The Chili RNA aptamer mimics large Stokes shift fluorescent proteins and exhibits high affinity for 3,5-dimethoxy-4-hydroxybenzylidene imidazolone (DMHBI) derivatives to elicit green or red fluorescence emission. The Chili RNA folds into a single coaxial helical stack with a length of ~70 Å that contains two A-form duplexes P1 and P2 that are separated by the central fluorophore binding domain (FBD). The P1 stem transitions via a base triple into a two-tiered G-quadruplex, which constitutes the core of the FBD. The ligand is immobilized by π-stacking between an unusual G14:G31 base pair and the T2 quartet.

Likewise, the structure of Chili–DMHBI+ was solved by MR and refined at a resolution of 2.95 Å. The crystallographic asymmetric unit (ASU) of the native datasets contained four copies of RNA-ligand complexes, which were superimposable with a root mean square deviation (rmsd) of 0.3 Å. The structural features of the DMHBO+ and DMHBI+ complexes are highly similar. In contrast to Spinach, which binds the deprotonated form of DFHBI, Chili exclusively binds the phenol form of DMHBI derivatives but enhances fluorescence of the phenolate forms. The positively charged groups in DMHBI+ and DMHBO+ substantially enhanced the binding affinity and fluorescence brightness. Time-correlated single photon counting (TCSPC) on the ns timescale revealed multiexponential decays for both Chili–DMHBO+ and Chili–DMHBI+ complexes but did not resolve the kinetics of proton transfer. Fluorescence and TA measurements on Chili–DMHBI+ gave a similar picture although with transient spectra shifted to shorter wavelengths. Again, proton transfer occurred in 120 fs. Preliminary 2D NMR experiments of the Chili–DMHBI+ complex in K+/Mg2+ solution revealed an unusual signal at a proton chemical shift of 8.6 ppm and 15N chemical shift of 142 ppm. The resonance unambiguously arises from an exchangeable proton of a guanine but does not belong to a shifted N1 imino proton of a canonical G:C Watson–Crick base pair.

>GGCUAGCUGGAGGGGCGCCAGUUCGCUGGUGGUUGGGUGCGGUCGGCUAGCC[4x]>[2x]AMKDLKG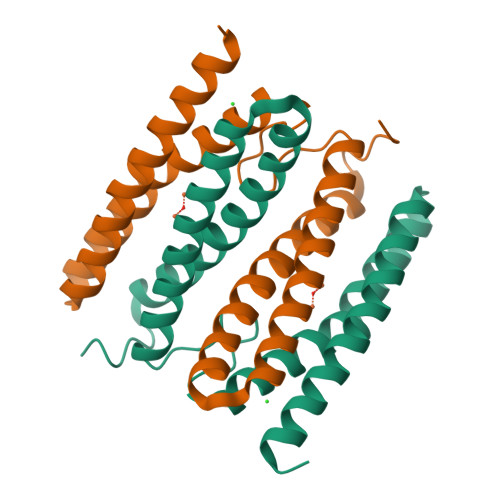TKTAENLKQGFIGESMANRRYLYFAKRADEEGYPEIAGLLRSIAEGETAHAFGHLDFIRQGGLTDPATDKPIGTLEQMIESAIAGETYEWTQMYPGFAKVAREEGFPEVAEWFETLARAEKSHAEKFQNVLKQLKGGT Here we use deep network hallucination to generate a wide range of symmetric protein homo-oligomers given only a specification of the number of protomers and the protomer length. Starting from only a choice of chain length L and oligomer valency N (2 for a dimer, 3 for a trimer, etc.), the method carries out a Monte Carlo search in sequence space starting from a random sequence. The loss function guiding the search is computed by inputting N copies of the sequence into the AlphaFold2 (AF2) network, and combining structure prediction confidence metrics (pLDDT; per-residue structural accuracy, and pTM; an estimate of the TM-score) with a measure of cyclic symmetry (the standard deviation of the distances between the center of mass of adjacent protomers within the predicted structure). To eliminate such over-fitting, we generated new sequences for the HAL backbones using the recently developed ProteinMPNN sequence design neural network (accompanying manuscript: Dauparas et al.).

To evaluate design accuracy we attempted crystallization of 19 designs and succeeded in solving crystal structures for seven (three C2s, two C3s and two C4s). All crystal structures had the correct oligomerization state and closely matched the design models (median Cα RMSD of 0.6 Å across all designs, with resolutions ranging from 1.8 to 3.4 Å). The side chain conformations in the crystal structures also closely match those of the design models. HALC2_068 is a fully helical dimer with an extensive interface formed by 6 interacting helices (3 from each protomer), with a single perpendicular helix buttressing the interfacial helices. Despite the low secondary structure complexity and absence of long-range contacts, this design also differs significantly from its closest structural relative in the PDB (TM-score: 0.57).

> MSGMIKVPEDLERIGRELRARGLDTKRLLEEGPKLYPELSIPDLMAIALYDHLNLDPEFLYRLLQQSRGS2-phenyl-N-{5-[(3R)-3-({5-[(phenylacetyl)amino]-1,3,4-thiadiazol-2-yl}oxy)pyrrolidin-1-yl]-1,3,4-thiadiazol-2-yl}acetamide 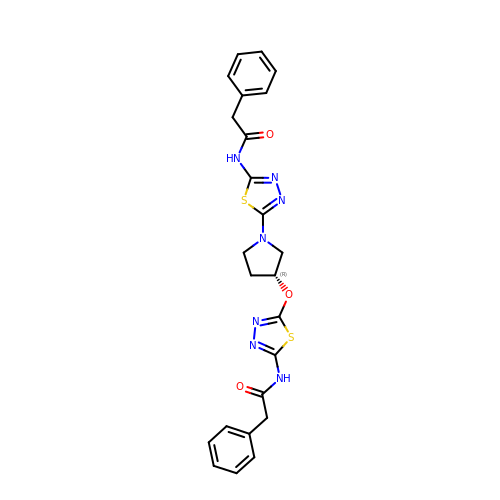| C24 H23 N7 O3 S2 | JGTIIKRXHSZCBG-GOSISDBHSA-N>[11x]GSHMGDFVVVYTDGCCSSNGRRRPRAGIGVYWGPGH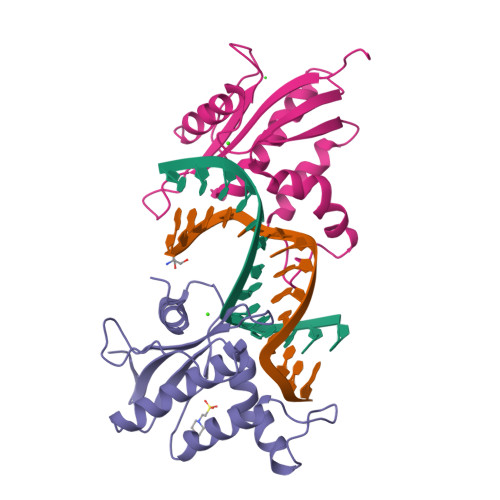PLNVGIRLPGRQTNQRAEIHAACKAIEQAKTQNINKLVLYTNSMFTINGITNWVQGWKKNGWKTSAGKEVINKEDFVALERLTQGMDIQWMHVPGHSGFIGNEEADRLAREGAKQSED>[4x]PCMLVALRPTNMDRERDKFFQSHYTYNPQFEYQEPMPTAVLEKYCEASGQFIHQAVGIIEAVLEKFGTYEHFEAATGGQLLTKCQIWSIVRKYMQKEGCAGEVVVQLSEDLLSQAVMMVENSRPTLAINLTGARQYWLEGMLRHEIGTHYLRGVNNARQP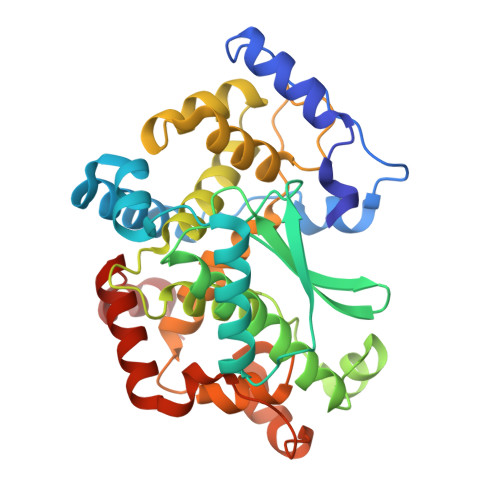WHNAEGRLRYGLRPANPTEEGLASLHSVLFRKQPFLWRAALLYYTIHRAARMSFRQLFQDLERYVQDADVRWEYCVRAKRGQTDTSLPGCFSKDQVYLDGIVRILRHRQTIDFPLLTSLGKVSYEDVDHLRPHGVLDNTRVPHFMQDLARYRQQLEHIMATNRLDEAELGRLLPD> SLHSSAQFDPILVADIGGTNARFALITAFDAAKNEFVIEYNHTFPSADFGSLQNATRHYLSTVPHIKPVRACLAVAGPIKAGQVHLTNLGWHFSVSEFKQAFSFLQLEVINDFAAFAYAAPYLDSNQNVVIKAGQADENSNIAVMGPGTGFGAACLVRTAQSSAVLSSEGGHISLAAVTDLDAKLLIELRKEHPHVSLETVFSGPGIAHLYKAMAAVNGITAKHLDAAQISNLANTGECEVCDATLNQFCDWLGSAAGDLALAYGALGGLFIGGGILPRMQSRLLESR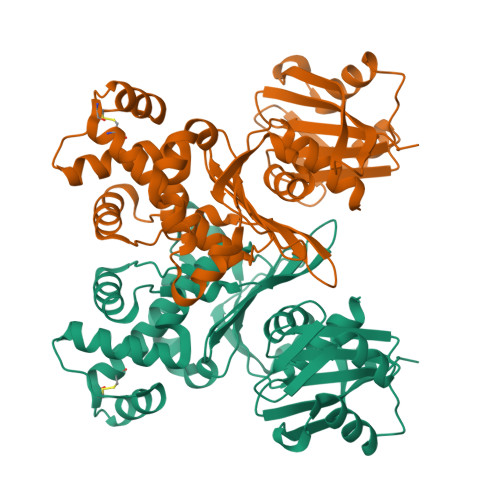FVERFSQKGIMSQYNGQVPVTLVTQDNIPLIGAAACLHNSKQE> MEEMPLRESSP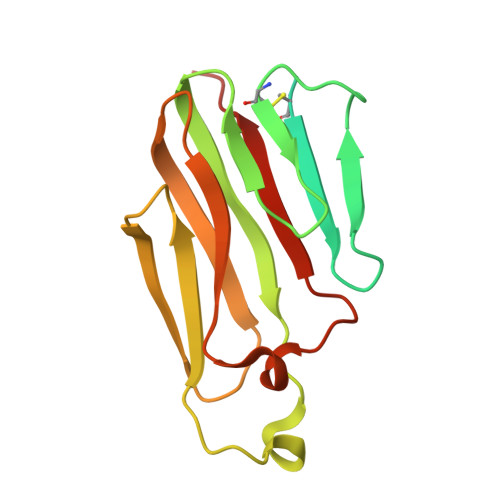QRAERCKKSWLLCIVALLLMLLCSLGTLIYTSLKPTAIESCMVKFELSSSKWHMTSPKPHCVNTTSDGKLKILQSGTYLIYGQVIPVDKKYIKDNAPFVVQIYKKNDVLQTLMNDFQILPIGGVYELHAGDNIYLKFNSKDHIQKTNTYWGIILMPDLPFIS>[2x]GHMSTLLINQPQYAWLKELGLREENEGVYNGSWGGRGEVITTYCPANNEPIARVRQASVADYEETVKKAREAWKIWADIPAPKRGEIVRQIGDALREKIQVLGSLVSLEMGKILVEGVGEVQEYVDICDYAVGLSRMIGGPILPSERSGHALIEQWNPVGLVG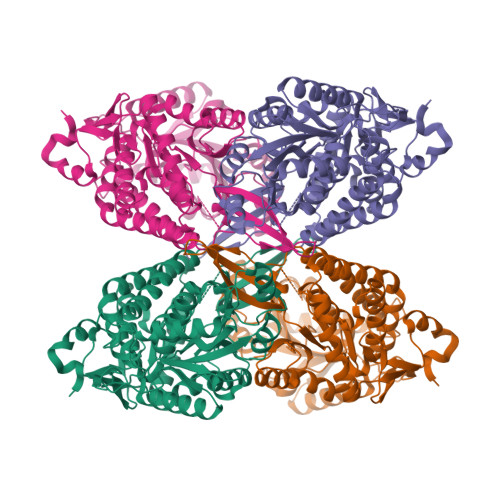IITAFNFPVAVYGWNNAIAMICGNVCLWKGAPTTSLISVAVTKIIAKVLEDNKLPGAICSLTCGGADIGTAMAKDERVNLLSFTGSTQVGKQVGLMVQERFGRSLLELGGNNAIIAFEDADLSLVVPSALFAAVGTAGQRCTTARRLFIHESIHDEVVNRLKKAYAQIRVGNPWDPNVLYGPLHTKQAVSMFLGAVEEAKKEGGTVVYGGKVMDRPGNYVEPTIVTGLGHDASIAHTETFAPILYVFKFKNEEEVFAWNNEVKQGLSSSIFTKDLGRIFRWLGPKGSDCGIVNVNIPTSGAEIGGAFGGEKHTGGGRESGSDAWKQYMRRSTCTINYSKDLPLAQGIKFQ> MKVQYCDSLVIGGGLAGLRAAVATQQKGLSTIVLSLIPVKRSHSAAAQGGMQASLGNSKMSDGDNEDLHFMDTVKGSDWGCDQKVARMFVNTAPKAIRELAAWGVPWTRIHKGDRMAIINAQKTTITEEDFRHGLIHSRDFGGTKKWRTCYTADATGHTMLFAVANECLKLGVSIQDRKEAIALIHQDGKCYGAVVRDLVTGDIIAYVAKGTLIATGGYGRIYKNTTNAVVCEGTGTAIALETGIAQLGNMEAVQFHPTPLFPSGILLTEGCRGDGGILRDVDGHRFMPDYEPEKKELASRDVVSRRMIEHIRKGKGVQSPYGQHLWLDISILGRKHIETNLRDVQEICEYF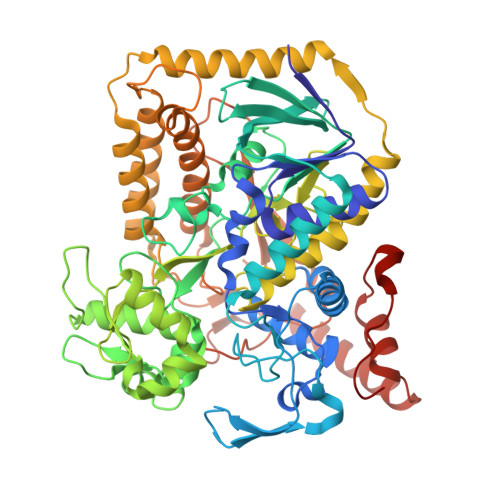AGIDPAEKWAPVLPMQHYSMGGIRTDYRGEAKLKGLFSAGEAACWDMHGFNRLGGNSVSEAVVAGMIVGEYFAEHCANTQVDLETKTLEKFVKGQEAYMKSLVESKGTEDVFKIKNRMKDVMDDNVGIFRDGPHLEKAVKELEELYKKSKNVGIKNKRLHANPELEEAYRVPMMLKVALCVAKGALDRTESRGAHNREDYPKRDDINWLNRTLASWPNPEQTLPTLEYEALDVNEMEIAPGYRGYGAKGNYIENPLSVKRQEEIDKIQSELEAAGKDRHAIQEALMPYELPAKYKARNERLGDKQRRR2-(3-bromophenyl)-8-fluoroquinoline-4-carboxylic acid | C16 H9 Br F 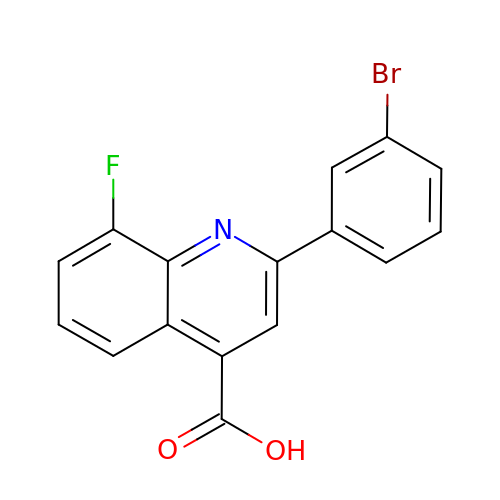N O2 | AONAJNHHHRKZDU-UHFFFAOYSA-N2,3-bis[[(Z)-octadec-9-enoyl]oxy]propyl (Z)-octadec-9-enoate | C57 H104 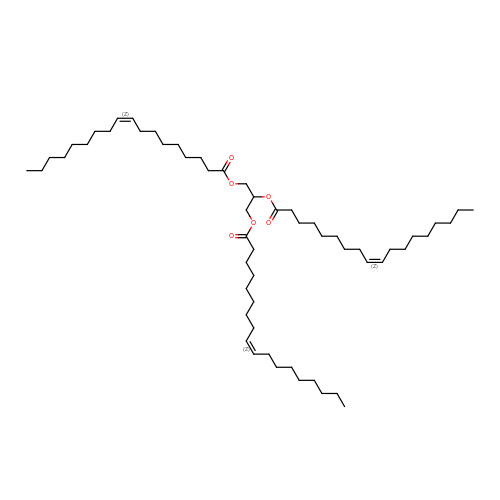O6 | PHYFQTYBJUILEZ-IUPFWZBJSA-N> GAMSDVSGFSMSSSAIARTETMTVLDDQYDQIINGYENYEEELEEDEEQN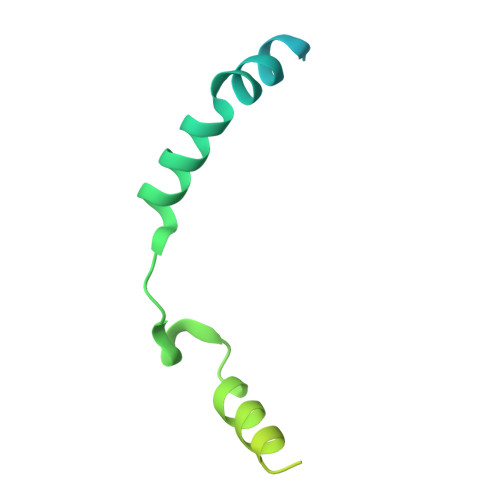YQPFDMSAERSDFESMLDDFLDNYELESGGRKLAKKDKEIERLKEAADEVSKGKLSQRRNRERQEKKKLEKVTNTLSSLKF> DYVLYKDATKPVEDRVADLLGRMTLAEKIGQMTQIERLVATPDVLRDNFIGSLLSGGGSVPRKGATAKEWQDMVDGFQKACMSTRLGIPMIYGIDAVHGQNNVYGATIFPHNVGLGATRDPYLVKRIGEATALEVRATGIQYAFAPCIAVCRDPRWGRCYESYSEDRRIVQSMTELIPGLQGDVPKDFTSGMPFVAGKNKVAACAKHFVGDGGTVDGINENNTIINREGLMNIHMPAYKNAMDKGVSTVMISYSSWNGVKMHANQDLVTGYLKDTLKFKGFVISDWEGIDRITTPAGSDYSYSVKASILAGLDMIMVPNKYQQFISILTGHVNGGVIPMSRIDDAVTRILRVKFTMGLFENPYADPAMAEQLGKQEHRDLAREAARKSLVLLKNGKTSTDAPLLPLPKKAPKILVAGSHADNLGYQCGGWTIEWQGDTGRTTVGTTILEAVKAAVDPSTVVVFAENPDAEFVKSGGFSYAIVAVGEHPYTETKGDNLNLTIPEPGLSTVQAVCGGVRCATVLISGRPVVVQPLLAASDALVAAWLPGSEGQGVTDALFGDFGFTGRLPRTWFKSVDQLPMNVGDAHYDPLFRLGYGLTTNATKKY

HvExoI releases a single Glc from non-reducing termini of oligo- and polymeric β-d-glucosides to support seed germination and plant development. HvExoI folds in an (α/β)8 barrel (domain 1) and an (α/β)6 sandwich (domain 2) that at their interface cradle a 13 Å-deep pocket- or crater-shaped active site. A vital conclusion drawn from the structural studies with the native β-d-glucan glucohydrolase, isoenzyme ExoI (HvExoI) isolated from barley seedlings, was that the glucose (Glc) product released from β-d-glucoside substrates remains entrapped in the enzyme active site until an incoming substrate binds, presumably lowering the energy barrier to facilitate Glc displacement. We discover that through chemical signalling, the incoming substrate evokes the formation of an autonomous and transient lateral cavity that serves as a conduit for the Glc product displacement from the active site.

To test the hypothetical Glc displacement route by using dGlc derivatives, crystals were perfused with saturating concentrations of 3dGlc and 4dGlc. The structures of both complexes showed that dGlc derivatives could not displace Glc from the −1 subsite, but that Glc consolidated to the −1 subsite. Others may argue that although most enzymes have evolved to use conformational adjustments to favour tight binding of correct substrates and product release, some enzymes may have not acquired this asset. This assumption was confirmed by perfusing dGlc derivatives that akin of reaction products could not remove Glc, but substrate analogues and mimics could.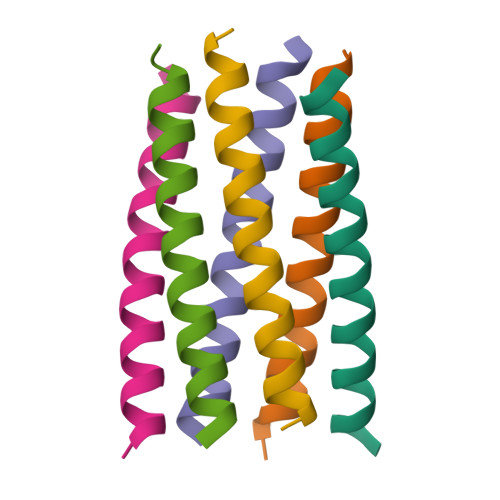>XGELAQALKELAKALKEEAWALKELAQALKGX[24x]>[3x]GCUGCUGC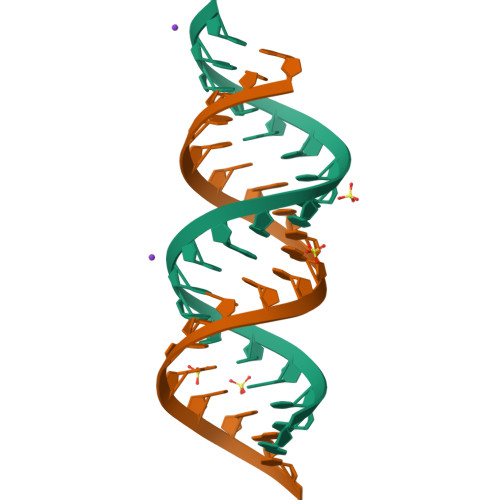UGCUGCUGCUGC> MRSKTLKKSLAAMYMRPPVTCYTDACEAPVAMWDGAIPLKETRKLKNGVPVRTVSRTYSHPPQLTPTQLSFNDINSMYCVGNDELIQFFPEGLGGRVFQTMPPGHPRGFLYRKETHLLNLFVDKVQHWHTKRSVLSSLTNGRTGFIVDGPTG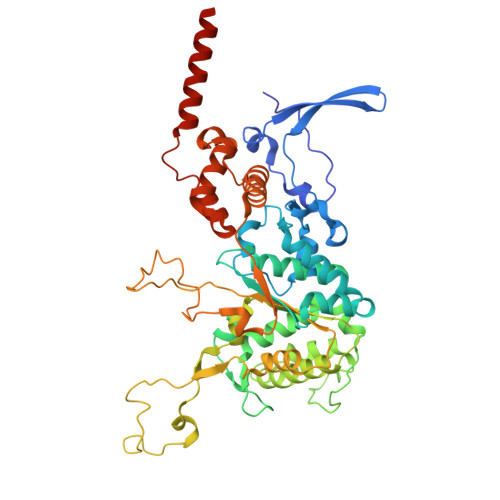CGKSALMCQVVHFARSRNIVTLYVPDAKVWTHGEWCWPSTILPGFFDAPDAARSFLKYFAVANRATLTSWKLRCTPKDLPTEQGERQPQNLYELCEWGHRAVAPASIDRQSVCVKFLMDELSEEKKLPVVIVVDGWNLFSHETHFRYPHPDFLRGLASFNESSTDIDLYPQELPRIPASRLSFVRGLNKMILSGDDPNKFFITCTTRDFKPFDGISGFPNVETDRFANSLDEYAPYDPEKDSHFHPIQIGNFDEYEYRSFLRFLINSGELAGLGWGPLWHASSDFERKLYKIGFLSGRNPQGVVDHYHQELVWRYDYQRTRQKQYLLKRRMEGMSRGASSGAVGVR>MGSSHHHHHHLVPRGSHMMSRSDQENPFIFKSNRFQTIYENENGHIRLLQRFDKRSKIFENLQNYRLLEYKSKPHTIFLPQFTDADFILVVLSGKAILTVLNSNDRNSFNLERGDTIKLPAGTIAYLANRDDNEDLRVLDLAIPVNRPGQLQSFLLSGTQNQPSFLSGFSKNILEAAFNTEYEEIEKVLLEEQEQKSQHRRSLRDKRQEITNEDVIVKVSREQIEELSKNAKSSSKKSVSSESEPFNLRSRNPIYSNKFGKFFEITPEKNPQLQDLDIFVNSVEIKEGSLLLPNYNSRAIVIVTVNEGKGDFELVGQRNENQQEQREENDEEEGQEEETTKQVQRYRARLSPGDVLVIPAGHPVAINASSDLNLIGFGI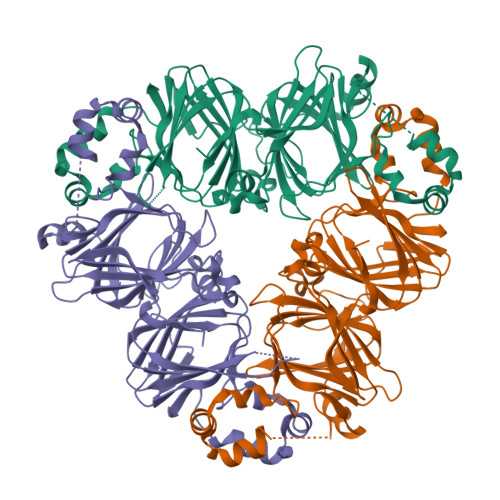NAKNNQRNFLAGEEDNVISQIQRPVKELAFPGSSREVDRLLTNQKQSHFANA[3x]[(2~{R},4~{a}~{R},6~{R},7~{a}~{R})-6-[2,4-bis(oxidanylidene)-5-(phosphonomethylsulfanylmethyl)pyrimidin-1-yl]-2-phenyl-4~{a},6,7,7~{a}-tetrahydro-4~{H}-furo[3,2-d][1,3]dioxin-2-yl]phosphonic 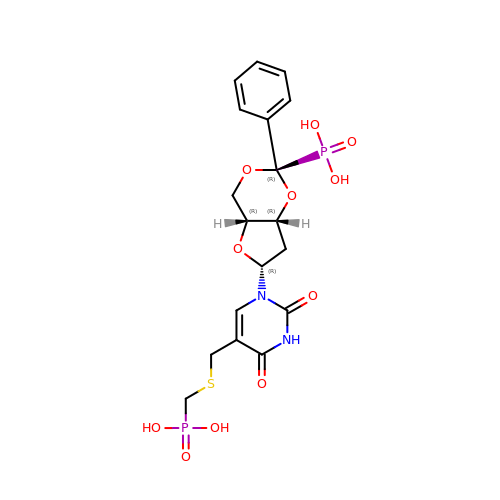acid | C18 H22 N2 O11 P2 S | KFRRWRABRKBEOD-ATNYBXOESA-N> MIDKSIMKKLLLTFLSIAAVCSLYAQRKVTQERMEQIYEEVKTPYKYGLAVAPTDNYHKIDCPTVFRQGDKWLMTYVVYNGKTGTDGRGYETWIAESDNLLDWRTLGRVLSYRDGKWDCNQRGGFPALPDMEWGGSYELQTYKGRHWMTYIGGEGTGYEAVKAPLFVGLASTKGDISTAHEWESLDKPILSIHDKDAQWWEKLTQYKSTVYWDKDKTLGAPFVMFYNAGGRHPETDLKGERVGIALSKDMKTWKRYPGNPVFAHEADGTITGDAHIQKMGDVYVMFYFSAFEPSRKYKAFNTFAASYDLVNWTDWHG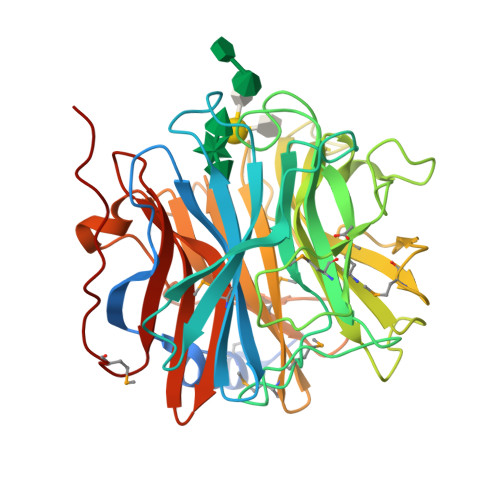ADLIIPSKNYDELFAHKSYVIKHDGVVYHFYCAVNNAEQRGIAIATSKPMGRSAVRFPKPETKN>MNHYEVLVLGGGSGGITMAARMKRKVGAENVAIVEPSERHFYQPIWTLVGAGAKQLSSSGRPTASVIPSGVEWIKARVTELNPDKNCIHTDDDEKISYRYLIIALGIQLDYEKIKGLPEGFAHPKIGSNYSVKTVEKTWKALQDFKEGNAIFTFPNTPVKCAGAPQKIMYLSEAYFRKTGKRSKANIIFNTSLGAIFGVKKYADALQEIIQERNLTVNYKKNLIEVRADKQEAVFENLDKPGETQVISYEMLHVTPPMSPPDVLKTSPVADAAGWVDVDKETLQ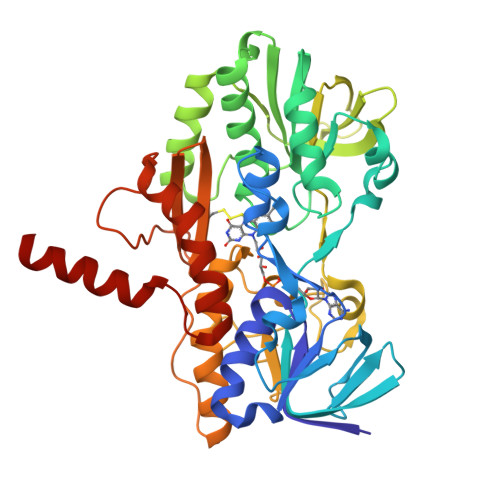HRRYPNVFGIGDCTNLPTSKTAAAVAAQSGILDRTISVIMKNQTPTKKYDGYTSCPLVTGYNRVILAEFDYKAEPLETFPFDQSKERLSMYLMKADLMPFLYWNMMLRGYWGGPAFLRKLFHLGMSLEH[4x]> LPLQPSSTMGQVG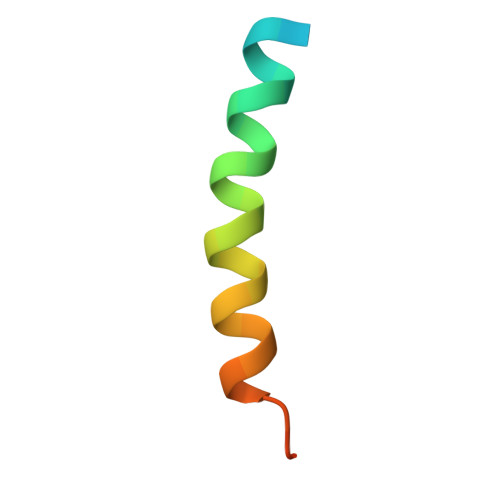RQLAIIGDDINRRYDSEFQTM> MRPPMYTSTNTEVPSRLVKNEHGSWQLIVNGKPFIMLAGELHNSSASTTEYLNSLWTSLKTLNLNTVLAPIAWEQFEPQEGIFDYTLINNMIDGARKNGFKLSILWFGSWKNGESSYAPTWVKEDTKRFFRVKSVEGKEIETISPFCENAMKADAKAFKTLVEHIKKVDQATGTVIALQPENEVGIFQGMDYSKASLAAYEQEVPQALIQYMKKNRKNLRKELLSVWEENGARTSGAWKTVFGDNAWSKSFYTTWQYATYIDFISAGAKEIYPLPTFCNCWLVQKPDDMPGVYPNGGPVSRVMDIWKAAAPHIDVLAPDIYLSDFKNIVADYHRADNPLLIPEAVMKPANAFWAFGEHSALCYSPFGIEDGADNFVFAQSYKVLNELIPLISEHQGSDRMIGVMKMPGESERTVTMGDYQLCIKYDAEDAYGLIIQTGKNEFVVAGINFKVYFTSTDKKKTGYIKQVWEGGYDTDGEWKATRLLNGDETYHNAVLIAKGRRTFTSEKSNNYNADHSDEIFVYSPTSYQAVWSPGIYRVTTYLRLEHHHHHH

In this study, we identify a β-galactosidase with novel substrate specificity from Bacteroides xylanisolvens, an intestinal bacterium. The gene encoding the Bxy_22780 protein in the GH35 family is a component of a gene cluster containing SusC-like and SusD-like proteins. In this study, we found that Bxy_22780 specifically hydrolyzes β-1,2-galactooligosaccharides. We propose β-1,2-galactooligosaccharide galactohydrolase as a systematic name and β-1,2-galactosidase as an accepted name for Bxy_22780.

To learn more about the binding modes of the natural substrates determined above, the ligand-free enzyme structure of the E350G mutant and the complex structures of the WT enzyme with galactose and methyl β-galactopyranoside (MeβGal) were determined at resolutions of 1.91, 1.86, and 1.94 Å, respectively. All the structures in this study were tetramers based on PISA server analysis, although the asymmetric units of these structures were found to contain two, one, and four molecules, respectively. The electron density of galactose in the α-anomer (α-Gal) configuration was clearly observed only at subsite −1 in the WT enzyme complex with α-Gal, whereas galactose in the β-anomer (β-Gal) configuration was not observed at all.> MNTGSFFINDEHDWQDVEPGIQRKIVAHTPDLMAVCVKFDRGAVGTPHQHERHDQIGYVVQGAFEVELEGEKRRLSPGDAFVAPHHTMHGAVALEPDSLVIDLFSP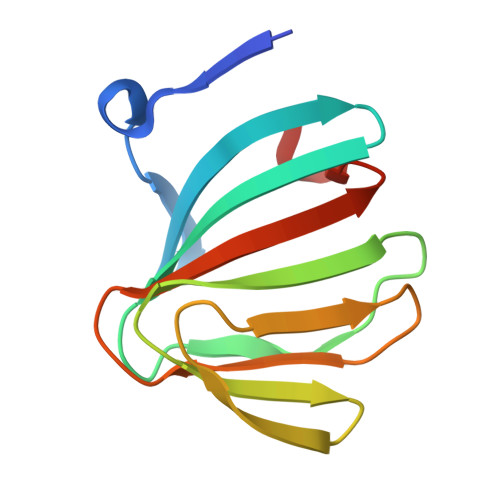RRDDMLKS> MSYSIDTLLLHNQYKHDSQTGAVNVPIYNTSTFHQFDVDTFGKYDYSRSGNPTREALEDIIALLEGGTKGFAFASGIAAISTAFLLLSQGDHVLISEDVYGGTYRVITEVLSRYGVSHTFVDMTNLEEIKQNIKPNTKLFYVETPSNPLLKVTDIREVSKLAKSIGALTFVDNTFLTPLFQKPLELGADVVLHSATKFIAGHSDVTAGLAVVKDSELAQKLGFLQNAFGAILGPQDCSLVLRGLKTLHVRLEHSAKNANKIAHYLQEHSKVKNVYYPGLQTHLGFDIQQSQATSAGAVLSFTLQSEDALRKFLSKVKLPVFAVSLGAVESILSYPAKMSHAALSQ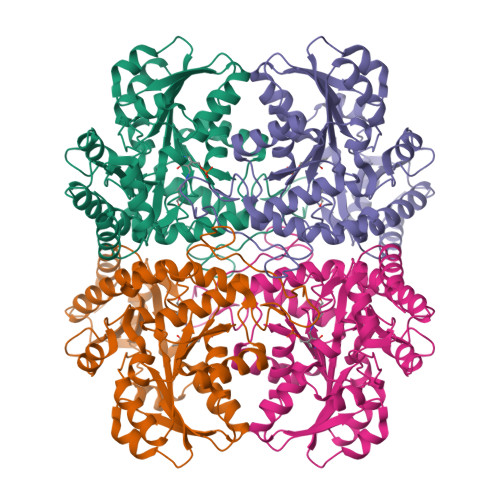EARDKRGISNSLLRLSVGLENVNDLISDFENALSYVEEPVNALEHHHHHH> GSETHRRVRLL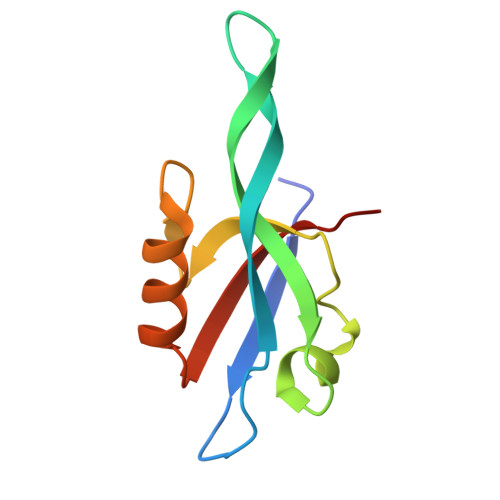KHGSDKPLGFYIRDGTSVRVTASGLEKQPGIFISRLVPGGLAESTGLLAVNDEVIEVNGIEVAGKTLDQVTDMMVANSSNLIITVKPANQR> GGNDRVRNLQSEVEGVKN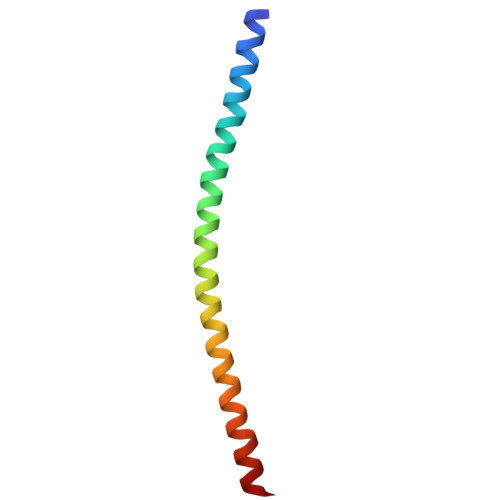IMTQNVERILARGENLEHLRNKTEDLEATSEHFKTTSQKVARKFWWKNVK> MQAGPA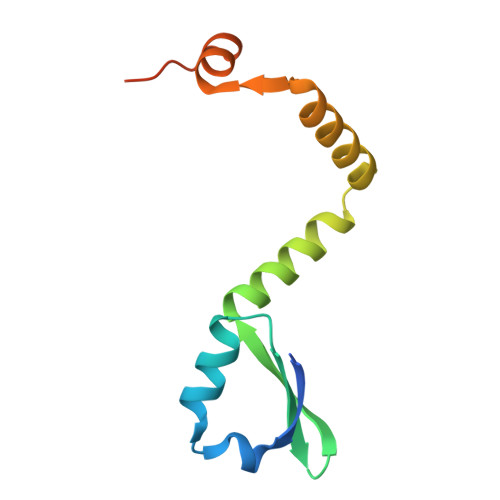LMRILPISTIKGKLNEFVDAVSSTQDQITITKNGAPAAVLVGADEWESLQETLYWLAQPGIRESIAEADADIASGRTYGEDEIRAEFGVPRRPHDYKDDDDK> MDIAIVDADNPADAIQQVKDLRKYGAKLIAYKSKSSEELKLALKAGADIAIVDADNPADAIQQVKDLRKYGAKLIAYKSKSSEELKLALKAGADIAIVDADNPADAIQQVKDLRKYGAKLIAYKSKSSEELKLALKAGADIAIVDADNPADAIQQVKDLRKYGAKLIAYKSKSSEELKLALKAGHHHHHH

Here, we investigate the capability of a deep neural network model to automate design of sequences onto protein backbones, having learned directly from crystal structure data and without any human-specified priors. To assess whether the model could perform sequence design for de novo structures, we tested our method on a Rosetta-generated four-fold symmetric de novo TIM-barrel backbone, a (βαβα)4 topology consisting of an eight-stranded barrel surrounded by eight alpha helices. We had the model fully redesign 50 four-fold symmetric sequences for the backbone and selected 8 designs for further characterization based on ranking by the model PLL and other metrics (see “Methods” section), using no information about previously confirmed sequences. Of these 8 designs, 4 are cooperatively folded proteins, as indicated by circular dichroism (CD) wavelength scans and by the presence of clear two-state transitions in thermal melt curves.

We successfully crystallized 2 model designs, F2C (1.46 Å resolution) and F15C (1.9 Å resolution), and the crystal structures validate that the sequences indeed fold into the TIM-barrel structure in agreement with the designed backbone. For F2C, the C-terminal helix is dislodged, although the complete barrel is formed. We hypothesize that the design of Ala3 (and symmetric positions Ala49, Ala95, Ala141) reduces the hydrophobic volume in the core, possibly allowing other interactions in the crystallization conditions to dislodge the helix (further discussion in Supplementary Note 1). In the structure, we see that the C-terminal His tag for F2C interacts with the surface of the beta-barrel, which might also contribute to the dislodging of the C-terminal helix, although 3 of the 4 symmetric subunits are folded as expected. A subset of these 8 structures was predicted to fold with low backbone deviation (<4 Å) into the target backbone by Rosetta (F2C, F4C) and trRosetta (F2C, F4C, F8C). For F2C, the model uses an isoleucine to wedge between the long and short helices and forming a Tyr-Glu-Ser polar network that extends to coordinate the loop from the beta-sheet to the short helix; for F15C, the model has a different solution, designing phenylalanine and valine residues (F10, V14) to pack the long helix against the shorter one near the top of the barrel. Particularly interesting are the Tyr-backbone contact and the His-Glu-backbone polar network for F2C and F15C, respectively, that help coordinate the helices across symmetric subunits at the base of the structure; these are the only hydrogen bonding solutions designed at this position among all previous structure-confirmed sequences for this scaffold.> MLICKVLKPLVSTNRIPGFEHKHLQVVLDGSSNKVAVDAVGCKPGDWVICVGSSAAREAAGSKSYPSDLTIVGIIDHWDPDSPKQIEV;>MGIALGMIETRGLVPAIEAADAMTKAAEVRLIGREFVGGGYVTVLVRGETGAVNAAVRAGADACERVGDGLVAAHIIARPHREVEPALGNGDFLGQKD[48x];>[2x]MSTKTSREIALERRKAMSDGGKKAALHSSSTKDRVRSSQDINSTGATSSNKKVLTSPSKSNIPANKIARKSTSSKLSSKELGIERRKAMSTHGKSAINSSDRTRTDVKSDIKVNKVISTEKPQALKDHNNNIKDNQVVKQNIKRRINQKRKPITNTSRDIVLARREAQSKHGKSASKQNTSAASLARRGDPDLSSREISQRVRELRSKTGSTSKQGNGKCRPCGPNKNGSKLNIADASWKVGKSETDSGQTVTGTQANRSLKTTGNEASTCRTVTGTQYMGAEVTGQFCQDKPKYKQPIRASVTTTTSGNKVTGNEVGRSEKVTGDEPGTCKNLTGTEYISANQSKKYCGEVIKKPSKVMQSITTDGLKVSGSLPGRSSLVTGDESGSGKQLTGDQYLGSEPSPKGKSFEKVGSYDTLNGNNVTGTGVGRSDYVTGNEYGSCKNLTGDEYIGSQQYEKFCGSTPKPEARKVGLSLSSKSNLISGTMTGRSKIVTGDEPGSCKVLTGTPYAGLDQINDNCNAEIADDMKSRATVNSGNNSNARLTGLQPGIGGVMTGATKGSCKNLTGTPYIGGDQFLSNCETPPNDASYANQEKSASNSWKEFSVNSPSREKYSAKNTEGVTGNRYEDSSKITGPFDMAEDKVTGTEQFRFEPNKNMTYKQKMKQEESQNIDIPTDKKEPSKITGEGQSAGNITGDDWDRGDKVTGTEGVSARKRNPSRAGFMGAMPPVDNKRN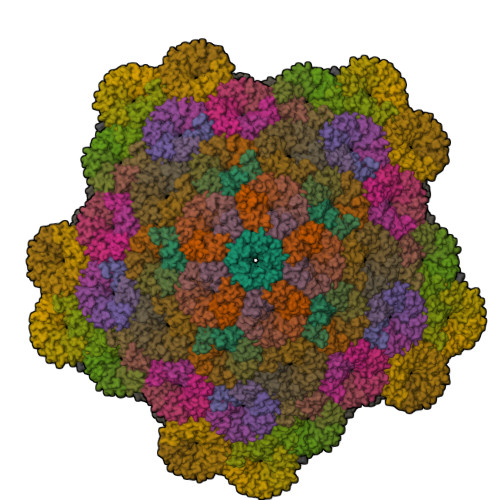DETEKPDFLITGSSGNTRDGQLVTFSGGARG>[4x]MGVKTFQFPFAEQLEKVAEQFPTFQILNEEGEVVNEEAMPELSDEQLKELMRRMVYTRILDQRSISLNRQGRLGFYAPTAGQEASQIASHFALEKEDFILPGYRDVPQIIWHGLPLYQAFLFSRGHFHGNQIPEGVNVLPPQIIIGAQYIQAAGVALGLKMRGKKAVAITYTGDGGTSQGDFYEGINFAGAFKAPAIFVVQNNRFAISTPVEKQTVAKTLAQKAVAAGIPGIQVDGMDPLAVYAAVKAARERAINGEGPTLIETLCFRYGPHTMSGDDPTRYRSKELENEWAKKDPLVRFRKFLEAKGLWSEEEENNVIEQAKEEIKEAIKKADETPKQKVTDLISIM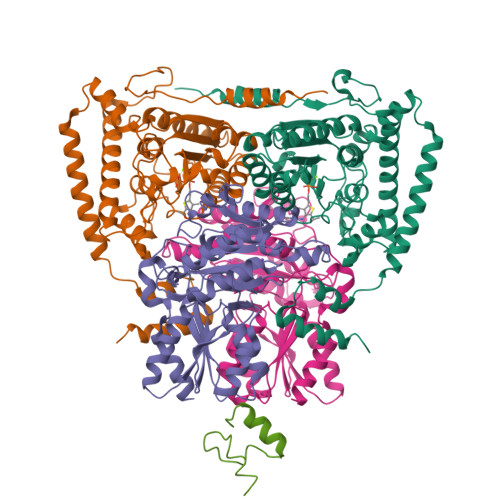FEELPFNLKEQYEIYKEKESK;>MAQMTMVQAITDALRIELKNDPNVLIFGEDVGVNGGVFRATEGLQAEFGEDRVFDTPLAESGIGGLAIGLALQGFRPVPEIQFFGFVYEVMDSICGQMARIRYRTGGRYHMPITIRSPFGGGVHTPELHSDSLEGLVAQQPGLKVVIPSTPYDAKGLLISAIRDNDPVIFLEHLKLYRSFRQEVPEGEYTIPIGKADIKREGKDITIIAYGAMVHESLKAAAELEKEGISAEVVDLRTVQPLDIETIIGSVEKTGRAIVVQEAQRQAGIAANVVAEINERAILSLEAPVLRVAAPDTVYPFAQAESVWLPNFKDVIETAKKVMNF[4x];>MAFEFKLPDIGEGIHEGEIVKWFVKPGDEVNEDDVLCEVQNDKAVVEIPSPVKGKVLEILVPEGTVATVGQTLITLDAPGYENMTFKGQEQEEAKKEEKTETVSKEEKVDAVAPNAPAAEAEAGPNRRVIAMPSVRKYAREKGVDIRLVQGTGKNGRVLKEDIDAFLAGGAKPAPAAAEEKAAPAAAKPATTEGEFPETREKMSGIRRAIAKAMVHSKHTAPHVTLMDEADVTKLVAHRKKFKAIAAEKGIKLTFLPYVVKALVSALREYPVLNTSIDDETEEIIQKHYYNIGIAADTDRGLLVPVIKHADRKPIFALAQEINELAEKARDGKLTPGEMKGASCTITNIGSAGGQWFTPVINHPEVAILGIGRIAEKPIVRDGEIVAAPMLALSLSFDHRMIDGATAQKALNHIKRLLSDPELLLMEA[2x]> MSMFNALNSNIEGEQYEAEEHSRELQIEQSFNILQDALIDLKNKDFEKSDSKFQELFQIDVVKPDRWGMYRNSSPTLDNLRYLCYRNRGMYYHLYLENNYERLNSQELVNCILKAVENLVESIQHSDADFAVTDLLARIFKSFNSVKLERLISEYEFTKQENLSLLLGRHRKFLLNDLTLMMNNYVELTNKLLVPNLSDNTIFERYHLEKYKDIKPEPLAFGPILSRISEMKKQDEEIMKKLDVFNVTLNEESWDEVAKALKNLLPSVKTSSLIGRNMDPYNEIEEPIEAVKFELSEAINNTPSLDRESERQEEEQDNESVRADDKSGNLAPSDIQTNEEARPNKRTDEHIDSTKPLQRSSKRFKEREQENSKELVMDVHKRFFGEFNTLLSYIHILPFCDFDTFASKFIIGSSDKQPEKFIPYTDLYECLKSWSSRYTDIFNQNDYLSSGSNENEELFQLNALLKSNAFDDKESFPRYLNDLDSDHIRSFISEVNAGNLHFHQVRLKLLFKLLGTYDEGNGRRLIIDYLWESQLLKIVLWFVFGIESNIFALINKNKRQCKYLALSIYELLVNHLGNIVEEITNKRIQGHKSADLKSQRNKVEKRIRSWHTLLEQIADEKDKELYVHFQWTHYCFLQYTCDIVDSRLSETLTSLENTIKDSDSSLDIAYPNYRHIPALNLNTVQSQKRKIRIIQNITVEDISEDTNSDTHSENHLETLEKVLLHILHPSTNHSNIDEEMVSFIFNSPFLLKIRLWGVLFSSYVKKSSIQDVQRIYFHVLDFMKGALTSPVYKESNPHGRHQMLLTVLTAIGYLSSQLTAILNSNRWESSDFVLEDYMFEKLLQTFFFFYTVLFYESSAVNDVSNKSFFKRASKSSGKMKDIMIDLATLILYYYDLQAKLRTPAEQGIETTELIWSLHTLFGHFHFCDASNGKFLDLAEKLLCQFINNDSFLQLKQILWCRYHYAIASDNFSPDLHDTKAVEMEKIHSLPLGTYLIKLQYQNKNPYLSSSKTTLKQIMDNIIEKIGDPSTLDNHIISRNSFLLNEYLSRPITADLLKHTFSGATSLYLTSPNDELQQGMTAGLFYVSSLQSLGLYKMRKKSMQARPSELDSIIRMLKNDIIYNTNRFESWILLGKCYSYIVEDDLIWTSDKITVPEKKDVIALTQRKAILCYLMAISIYYSKLDRTIDDKKIILEALDDLGSMLISGYYNPMNKLCFSWKSSAENTMRLSETGEVVMEKTKKITTISD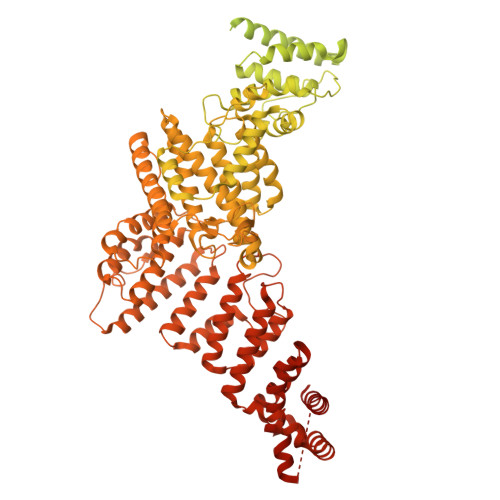FNIEQSIFLCFNRACSLSGDIKSQDDVFVLNWSSFYNLAKFFFKTDGGNNCKLVAKYITQGCQIAYESSPAKDPIIEPHYLLVNACYKWVKRGVIGVNEALTLLSKDNQFFQEQEEFWVNDEGLAWDYQEKFFFDKIIRLLRHLLSVDKKKWQHRPRYRIARILFDDLGDVNGALEEMDSLISAKSINKNLVNIWKPDFERPGKHFIYTYQYLVLYLDLLFAIKDFNTTGLVIKKLRRFGSGTVNVNELLERAINVYTQSAKIKLQLQDKSYVEQILPTLNYQEFLKISEQLNQVFDQGKYPEEISSGLKLAFQLKKGHSGIAFDSVCLGIYFEYLYFPLARQDQSLTDVNDENNPALPSSGSVTSKSTPDPTSKPSAIKKRVTKKEVFDRVRLLVDKIT> GMVRISIAGGNEIDPGSMGLTLFHEHLRLITEVVRWNWPHLYNEDEELKRAIDAVNAAKKYGVKTIIDLTVAGIGCDVRFNEKVAKATGVNIIMGTGFYTYTEIPFYFKNRGIDSLVDAFVHDITIGIQGTNTRAAFVKA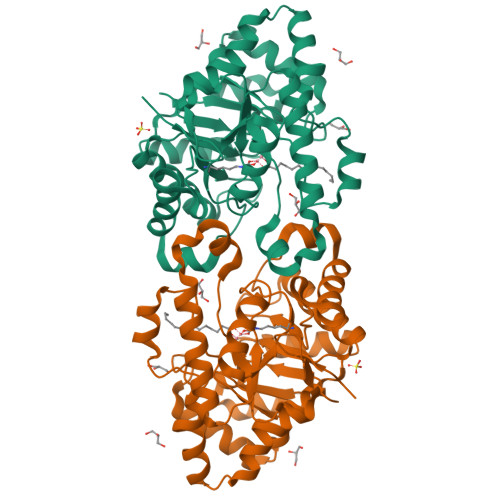VIDSSGLTKDVEMAIRAAAKAHIKTDVPIITHSFVGNKSSLDLIRIFKEEGVDLARTVIGHVGDTDDISFIEQILREGAFIGLDRFGLDIYLPLDKRVKTAIELIKRGWIDQLLLSHDYCPTIDWYPPEVVRSTVPDWTMTLIFEKVIPRMRSEGITEEQINRVLIDNPRRLFTGR> MADLAECNIKVMCRFRPLNESEVNRGDKYIAKFQGEDTVVIASKPYAFDRVFQSSTSQEQVYNDCAKKIVKDVLEGYNGTIFAYGQTSSGKTHTMEGKLHDPEGMGIIPRIVQDIFNYIYSMDENLEFHIKVSYFEIYLDKIRDLLDVSKTNLSVHEDKNRVPYVKGCTERFVCSPDEVMDTIDEGKSNRHVAVTNMNEHSSRSHSIFLINVKQENTQTEQKLSGKLYLVDLAGSEKVSKTGAEGAVLDEAKNINKSLSALGNVISALAEGST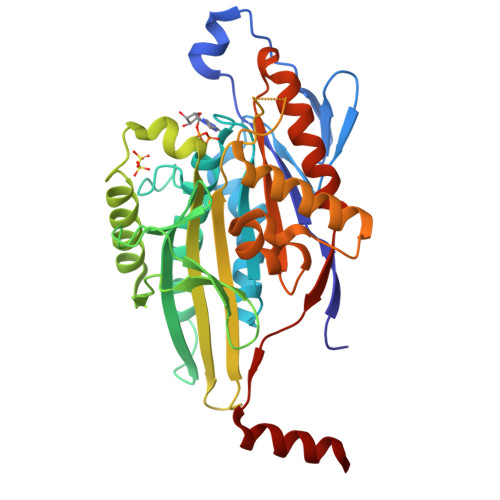YVPYRDSKMTRILQDSLGGNCRTTIVICCSPSSYNESETKSTLLFGQRAKTIKNTVCVNVELTAEQWKKKYEKEKE Complex I (NADH:ubiquinone (UQ) oxidoreductase) is the first and the largest enzyme of the respiratory chain, catalysing the transfer of two electrons from NADH to UQ, coupled to the translocation of four protons across the bacterial or inner mitochondrial membrane. In bacterial complex I the 14 “core” subunits, necessary and sufficient for complex I function, are shared equally between the peripheral and membrane arms, together forming an L-shaped molecule. All known co-factors of complex I reside in the PA: the primary electron acceptor flavin-mononucleotide (FMN) is connected by the redox chain of seven Fe–S clusters to the quinone-binding site (Q-site) at the interface with the membrane domain. In this work we address this question by building and analyzing atomic structures of nine different conformational states of complex I, which were obtained by X-ray crystallography and single-particle cryo-EM.

Aureothin, pyridaben and piericidin A are the most potent inhibitors of T. thermophilus complex I, while rotenone is less effective than it is with mammalian enzyme. All Q-like ligands studied here display a similar pattern of interactions at the deepest end of the Q-cavity, with the headgroup about 12 Å away from cluster N2. A shared feature between all ligands bound in the Q-site is a hydrogen bond interaction of a ketone group from the quinone ring with the conserved and essential for complex I activity Y87416,36. In the case of aureothin, H384 stabilizes its outer ether group, while M516 interacts with the oxygen in the furanose ring. The distal nitrobenzene moiety is surrounded by both charged and nonpolar residues that, despite the lack of direct interaction, might form a suitable pocket for its accommodation. In these structures quinone-like compounds are bound in the main “deep” site within the cavity, where quinone can effectively accept electrons from cluster N2. Most dramatic changes are caused by DQ binding, whilst Q-like inhibitors alter complex I conformation consistently in a similar way but to a lesser degree, to states intermediate between CXIINT and CXIDQ. The overlap analysis (OA) (technique described below) shows that transitions from CXIINT structure to CXIAUT and CXIPYR involve relatively minor PA rotation component (mode 8), which is much stronger for CXIPIE structure and is accompanied in addition by a bending motion (mode 7) for CXIDQ structure.

>[2x]MTGPILSGLDPRFERTLYAHVGKEGSWTLDYYLRHGGYETAKRVLKEKTPDEVIEEVKRSGLRGRGGAGFPTGLKWSFMPKDDGKQHYLICNADESEPGSFKDRYILEDVPHLLIEGMILAGYAIRATVGYIYVRGEYRRAADRLEQAIKEARARGYLGKNLFGTDFSFDLHVHRGAGAYICGEETALMNSLEGLRANPRLKPPFPAQSGLWGKPTTINNVETLASVVPIMERGADWFAQMGTEQSKGMKLYQISGPVKRPGVYELPMGTTFRELIYEWAGGPLEPIQAIIPGGSSTPPLPFTEEVLDTPMSYEHLQAKGSMLGTGGVILIPERVSMVDAMWNLTRFYAHESCGKCTPCREGVAGFMVNLFAKIGTGQGEEKDVENLEALLPLIEGRSFCPLADAAVWPVKGSLRHFKDQYLALAREKRPVPRPSLWR;>[2x]MGFFDDKQDFLEETFAKYPPEGRRAAIMPLLRRVQQEEGWIRPERIEEIARLVGTTPTEVMGVASFYSYYQFVPTGKYHLQVCATLSCKLAGAEELWDYLTETLGIGPGEVTPDGLFSVQKVECLGSCHTAPVIQVNDEPYVECVTRARLEALLAGLRAGKRLEEIELPGKCGHHVHEVEV;>MVRVKVNDRIVEVPPGTSVMDAVFHAGYDVPLFCSEKHLSPIGACRMCLVRIGLPKKGPDGKPLLNEKGEPEIQWQPKLAASCVTAVADGMVVDTLSDVVREAQAGMVEFTLLNHPLDCPTCDKGGACELQDRTVEYGLYEKYYQKGPLELPVYTRFEFTRRHVDKHHPLSPFVILDRERCIHCKRCVRYFEEVPGDEVLDFIERGVHTFIGTMDFGLPSGFSGNITDICPVGALLDLTARFRARNWEMEETPTTCALCPVGCGITADTRSGELLRIRAREVPEVNEIWICDAGRFGHEWADQNRLKTPLVRKEGRLVEATWEEAFLALKEGLKEARGEEVGLYLAHDATLEEGLLASELAKALKTPHLDFQGRTAAPASLFPPASLEDLLQADFALVLGDPTEEAPILHLRLSEFVRDLKPPHRYNHGTPFADLQIKERMPRRTDKMALFAPYRAPLMKWAAIHEVHRPGEEREILLALLGDKEGSEMVAKAKEAWEKAKNPVLILGAGVLQDTVAAERARLLAERKGAKVLAMTPAANARGLEAMGVLPGAKGASWDEPGALYAYYGFVPPEEALKGKRFVVMHLSHLHPLAERYAHVVLPAPTFYEKRGHLVNLEGRVLPLSPAPIENGEAEGALQVLALLAEALGVRPPFRLHLEAQKALKARKVPEAMGRLSFRLKELRPKERKGAFYLRPTMWKAHQAVGKAQEAARAELWAHPETARAEALPEGAQVAVETPFGRVEARVVHREDVPKGHLYLSALGPAAGLRVEGRVLVPAGGEA[2x];>MREEFLEEIPLDAPPEEAKELRTEVMTLNVGPQHPSTHGVLRLMVTLSGEEVLEVVPHIGYLHTGFEKTMEHRTYLQNITYTPRMDYLHSFAHDLAYALAVEKLLGAVVPPRAETIRVILNELSRLASHLVFLGTGLLDLGALTPFFYAFRERETILDLFEWVTGQRFHHNYIRIGGVKEDLPEEFVPELKKLLEVLPHRIDEYEALFAESPIFYERARGVGVIPPEVAIDLGLTGGSLRASGVNYDVRKAYPYSGYETYTFDVPLGERGDVFDRMLVRIREMRESVKIIKQALERLEPGPVRDPNPQITPPPRHLLETSMEAVIYHFKHYTEGFHPPKGEVYVPTESARGELGYYIVSDGGSMPYRVKVRAPSFVNLQSLPYACKGEQVPDMVAIIASLDPVMGDVDR[2x];>[2x]MRLERVLEEARAKGYPIEDNGLGNLWVVLPRERFKEEMAHYKAMGFNFLADIVGLDYLTYPDPRPERFAVVYELVSLPGWKDGDGSRFFVRVYVPEEDPRLPTVTDLWGSANFLEREVYDLFGIVFEGHPDLRKILTPEDLEGHPLRKDYPLGETPTLFREGRYIIPAEFRAALTGKDPGLTFYKGGSRKGYRSLWADLKKAREVKG;>[2x]MALKDLFERDVQELEREGILFTTLEKLVAWGRSNSLWPATFGLACCAIEMMASTDARNDLARFGSEVFRASPRQADVMIVAGRLSKKMAPVMRRVWEQMPDPKWVISMGACASSGGMFNNYAIVQNVDSVVPVDVYVPGCPPRPEALIYAVMQLQKKVRGQAYNERGERLPPVAAWKRTRG;>[2x]MSASSERELYEAWVELLSWMREYAQAKGVRFEKEADFPDFIYRMERPYDLPTTIMTASLSDGLGEPFLLADVSPRHAKLKRIGLRLPRAHIHLHAHYEPGKGLVTGKIPLTKERFFALADRAREALAFA;>MTLKALAQSLGITLKYLFSKPVTVPYPDAPVALKPRFHGRHVLTRHPNGLEKCIGCSLCAAACPAYAIYVEPAENDPENPVSAGERYAKVYEINMLRCIFCGLCEEACPTGAIVLGYDFEMADYEYSDLVYGKEDMLVDVVGTKPQRREAKRTGKPVKVGYVVPYVRPELEGFKAPTEGGKR[2x];>MAPIQEYVGTLIYVGVALFIGVAALLVGALLGPKKPGRAKLMPYESGNDPAGEVKRFPVHFYVVAMLFILFDVEVAFLWPYAVSAGGLGLYGFLGVLAFTLLLFVGFLYEWWKGVMRWH[2x];>MTWSYPVDPYWMVALKALLVVVGLLTAFAFMTLIERRLLARFQVRMGPNRVGPFGLLQPLADAIKSIFKEDIVVAQADRFLFVLAPLISVVFALLAFGLIPFGPPGSFFGYQPWVINLDLGILYLFAVSELAVYGIFLSGWASGSKYSLLGSLRSSASLISYELGLGLALLAPVLLVGSLNLNDIVNWQKEHGWLFLYAFPAFLVYLIASMAEAARTPFDLPEAEQELVGGYHTEYSSIKWALFQMAEYIHFITASALIPTLFLGGWTMPVLEVPYLWMFLKIAFFLFFFIWIRATWFRLRYDQLLRFGWGFLFPLALLWFLVTALVVALDLPRTYLLYLSALSFLVLLGAVLYTPKPARKGGGA[2x];>MSLLEGLALFLLLLSGVLVVTLRNAIHAALALILNFLVLAGVYVALDARFLGFIQVIVYAGAIVVLFLFVIMLLFAAQGEIGFDPLVRSRPLAALLALGVAGILAAGLWGLDLAFTQDLKGGLPQALGPLLYGDWLFVLLAVGFLLMAATVVAVALVEPGKASRAKEAEKREEVAR[2x];>[2x]MSYLLTSALLFALGVYGVLTRRTAILVFLSIELMLNAANLSLVGFARAYGLDGQVAALMVIAVAAAEVAVGLGLIVAIFRHRESTAVDDLSELRG;>[2x]MALLGTILLPLLGFALLGLFGKRMREPLPGVLASGLVLASFLLGAGLLLSGGARFQAEWLPGIPFSLLLDNLSGFMLLIVTGVGFLIHVYAIGYMGGDPGYSRFFAYFNLFIAMMLTLVLADSYPVMFIGWEGVGLASFLLIGFWYKNPQYADSARKAFIVNRIGDLGFMLGMAILWALYGTLSISELKEAMEGPLKNPDLLALAGLLLFLGAVGKSAQIPLMVWLPDAMAGPTPVSALIHAATMVTAGVYLIARSSFLYSVLPDVSYAIAVVGLLTAAYGALSAFGQTDIKKIVAYSTISQLGYMFLAAGVGAYWVALFHVFTHAFFKALLFLASGSVIHALGGEQDVRKMGGLWKHLPQTRWHALIGALALGGLPLLSGFWSKDAILAATLTYPFGGVGFYVGALLVAVLTAMYAMRWFVLVFLGEERGHHHPHEAPPVMLWPNHLLALGSVLAGYLALPHPLPNVLEPFLKPALAEVEAHHLSLGAEWGLIALSAAVALLGLWAGFVFFQRKVFPAWYLAFEAASREAFYVDRAYNALIVNPLKALAEALFYGDRGLLSGYFGLGGAARSLGQGLARLQTGYLRVYALLFVLGALLLLGVMRW;>[2x]MVVLAVLLPVVFGALLLLGLPRALGVLGAGLSFLLNLYLFLTHPGGVAHAFQAPLLPGAGVYWAFGLDGLSALFFLTIALTVFLGALVARVEGRFLGLALLMEGLLLGLFAARDLLVFYVFFEAALIPALLMLYLYGGEGRTRALYTFVLFTLVGSLPMLAAVLGARLLSGSPTFLLEDLLAHPLQEEAAFWVFLGFALAFAIKTPLFPLHAWLPPFHQENHPSGLADALGTLYKVGVFAFFRFAIPLAPEGFAQAQGLLLFLAALSALYGAWVAFAAKDFKTLLAYAGLSHMGVAALGVFSGTPEGAMGGLYLLAASGVYTGGLFLLAGRLYERTGTLEIGRYRGLAQSAPGLAALALILFLAMVGLPGLSGFPGEFLTLLGAYKASPWLAALAFLSVIASAAYALTAFQKTFWEEGGSGVKDLAGAEWGFALLSVLALLLMGVFPGYFARGLHPLAEAFAKLLGGGA;>MTLAILAVFSVALTLLGFVLPPQGVKRATLLGLALALASLLLTWGKPFAFGPYAVDGVSQVFTLLALLGALWTVGLVRSGRFEFYLLVLYAALGMHLLASTRHLLLMLVALEALSLPLYALATWRRGQGLEAALKYFLLGALAAAFFLYGAALFYGATGSLVLGAPGEGPLYALALGLLLVGLGFKAALAPFHFWTPDVYQGSPTPVVLFMATSVKAAAFAALLRVAAPPEALALLVALSVVVGNLAALAQKEAKRLLAYSSIAHAGYMALALYTGNAQALGFYLLTYVLATGLAFAVLSQISPDRVPLEALRGLYRKDPLLGLAFLVAMLSLLGLPPLAGFWGKYLAFAEAARAGAWGVLVLALVTSAVSAYYYLGLGLAVFARPEETPFRPGPPWARAAVVAAGVLLLALGLLPGLVLPALAAGG[2x];>[2x]MVRVGMRAAPRVSLEALKAALGGLKLSEAKVYLITDWQDKRDQARYALLLHTGKKDLLVPDAFGPAFPGGEEALSELVGLLLAQGARRFYEAVVSPGEMTALLDLPPEELLKRVMAIANPTDPGIYLKRAA>SNANTPQEAQQVDMWKKYIQWEKSNPLRTEDQTLITKRVMFAYEQCLLVLGHHPDIWYEAAQYLEQSSKLLAEKGDMNNAKLFSDEAANIYERAISTLLKKNMLLYFAYADYEESRMKYEKVHSIYNRLLAIEDIDPTLVYIQYMKFARRAEGIKSGRMIFKKAREDTRTRHHVYVTAALMEYYCSKDKSVAFKIFELGLKKYGDIPEYVLAYIDYLSHLNEDNNTRVLFERVLTSGSLPPEKSGEIWARFLAFESNIGDLASILKVEKRRFTAFKEEYEGKETALLVDRYKFMDLYPCSASELKALGYKDV[2x];>SNAMSAGEVERLVSELSGGTGGDEEEE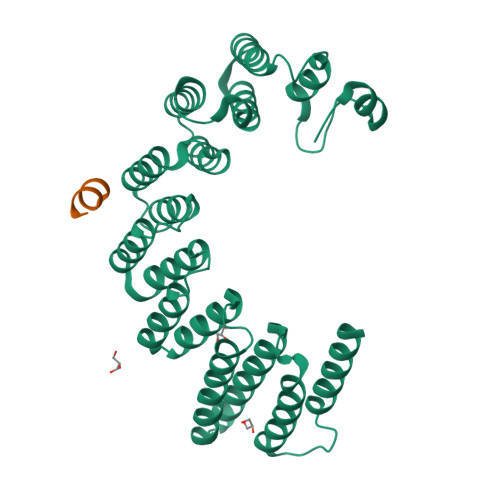WLYGDENEVER[2x]>[2x]MEEEAAVE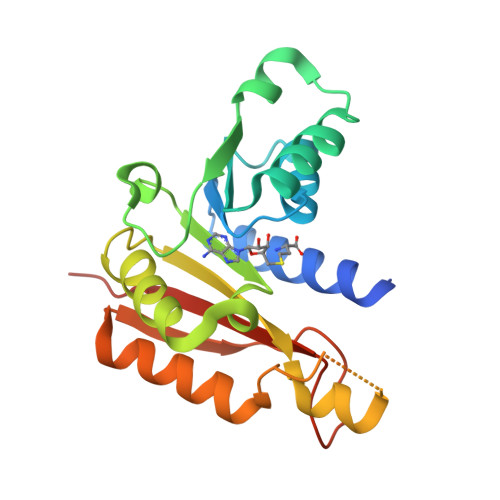KPISLNQQRMNGVVAALKQSNARRVIDLGCGQGNLLKILLKDSFFEQITGVDVSYRSLEIAQERLDRLRLPRNQWERLQLIQGALTYQDKRFHGYDAATVIEVIEHLDLSRLGAFERVLFEFAQPKIVIVTTPNIEYNVKFANLPAGKLRHKDHRFEWTRSQFQNWANKITERFAYNVQFQPIGEADPEVGSPTQMAVFIHRGHHHHHH>MHHHHHHMSSKQFKILVNEDYQVNVPSLPIRDVLQEIKYCYRNGFEGYVFVPEYCRDLVDCDRK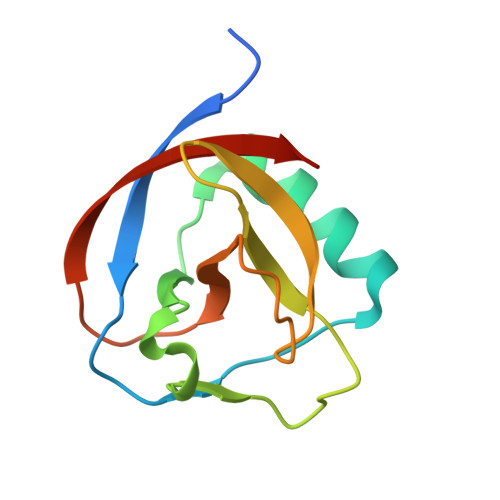DHYVIGVLGNGVSDLKPVLLTEPSVMLQGFIVRANCNGVLEDFDLKIARTGR[4x]(2Z)-3-{[OXIDO(OXO)PHOSPHINO]OXY}-2-PHENYLACRYLATE 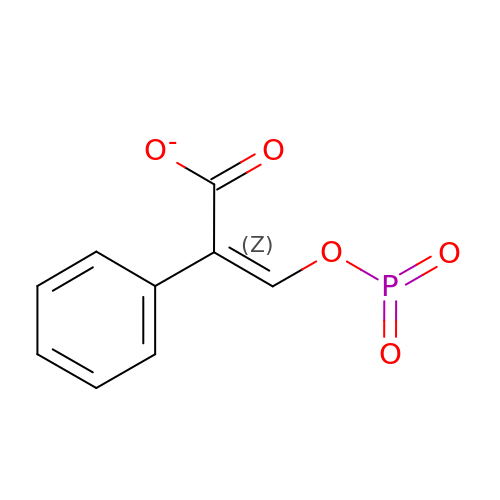| C9 H6 O5 P | WSMRUPUEYOBWRC-VURMDHGXSA-M> AQKLVFFAAAIIGLM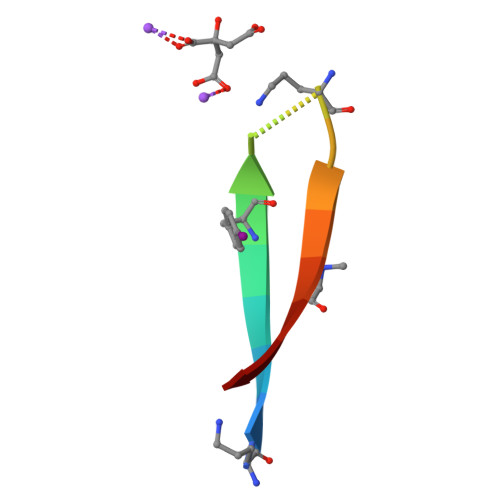V> FSDGVTAMGFQSLDTQVSIKDILRRPVLLFNHVELDPDYTGFFIPIMPPSRMMQYKSGDKETSFQRLIGRTPQAAIMNLFRFWRGSLRYTIIIHSTDGHPIYVTHVPHTGNRVYGLMKVN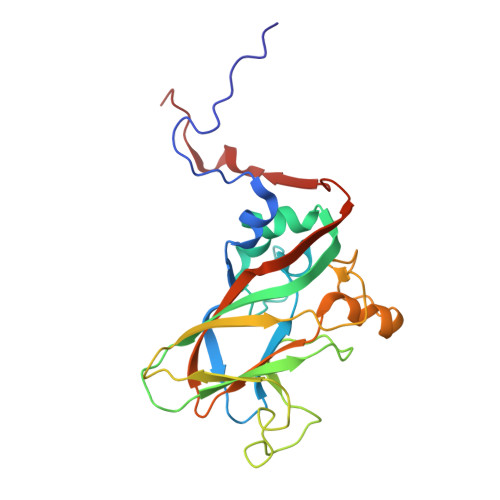NLHEYTKVPIFGCGLTTEMIIPSVNPSICVEVPFDTENNWAVTFDEDAQRNYSWRDKGDTVTGHLVVTPVVSVYMSVWVEAGDDFEVSNFYGPPSVKTNDWNYAFSDEH> GDLADRFAELERRYDARLGVYVPATGTTEAIEYRADERFAFCSTFKAPLVAAVLHQNPLTHLDK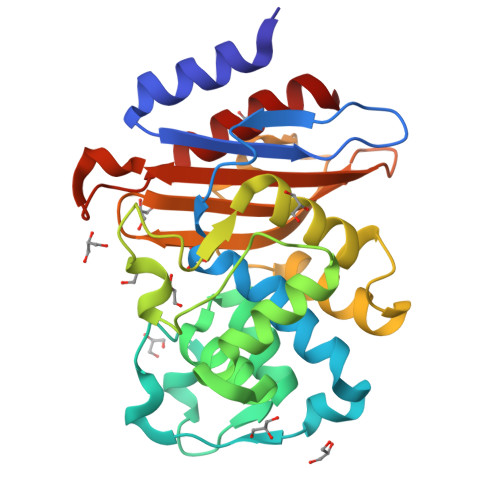LITYTSDDIRSISPVAQQHVQTGMTIGQLCDAAIRYSDGTAANLLLADLGGPGGGTAAFTGYLRSLGDTVSRLDAEEPELNRDPPGDERDTTTPHAIALVLQQLVLGNALPPDKRALLTDWMARNTTGAKRIRAGFPADWKVIDKTGTGDYGRANDIAVVWSPTGVPYVVAVMSDRAGGGYDAEPREALLAEAATCVAGVLA>GLVPRGSEDKWRNAFDHMLMEEFEEKMDQIEHGLLMLSEQYKELEKTKSKELKEQILRELTIAENYLRGALKFMQQEAKRTDLNMFERYNF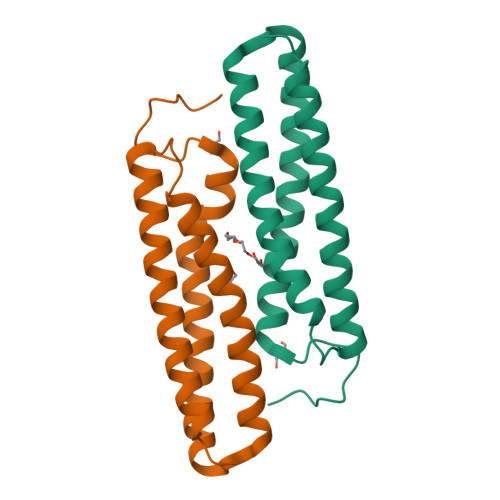ETAVSTIEILVKDLAELAKKVKAVKSD[2x]> SNADRRERTLASQSVNKYILSIQDIYKNSPVPVCVRNQSRKIIYANGAFIELFSKEDQPLSGDSYNRYGVEVFLSSLELECQSLGHGAAFCRRFNFHGEIYQIRMENISFDNNEIIVLW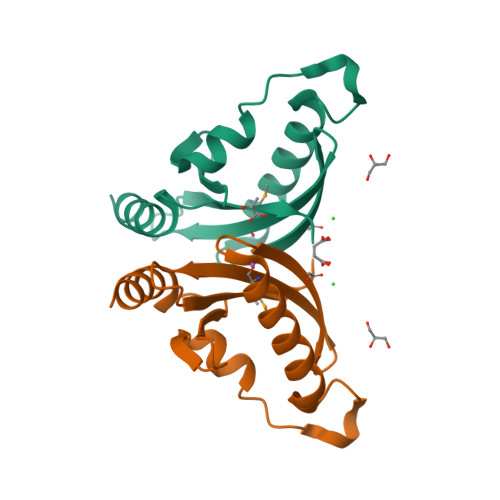QINLFPDH>[10x]MSRPPPPRAASGAPLRPATVLGTMEMGRRMDASASAASVRAFLERGHSELDTAFMYCDG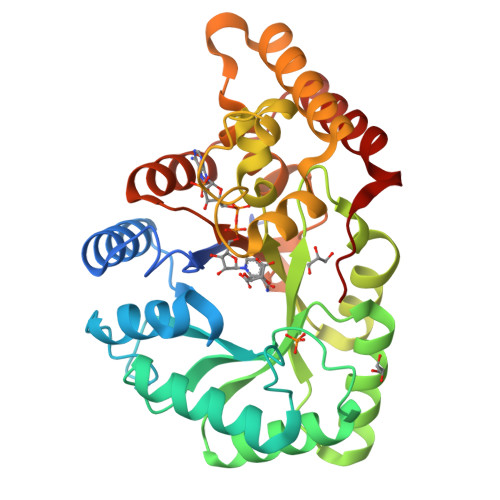QSENILGGLGLGLGSGDCTVKIATKANPWEGKSLKPDSIRSQLETSLKRLQCPRVDLFYLHAPDHSTPVEETLCACHQLHQEGKFVELGLSNYASWEVAEICTLCKSNGWILPTVYQGMYNATTRQVEAELLPCLRHFGLRFYAYNPLAGGLLTGKYKYEDKDGKQPVGRFFGNNWAETYRNRFWKEHHFEAIALVEKALQTTYGTNAPRMTSAALRWMYHHSQLQGTRGDAVILGMSSLEQLEQNLAATEEGPLEPAVVEAFDQAWNMVAHECPNYFR> YAEHKSHRGEVSVCDSESLWVTDKSS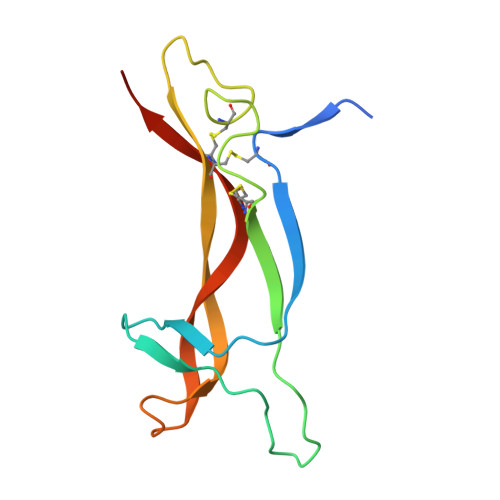AIDIRGHQVTVLGEIKTQNSPVKQYFYETRCKEARPVKNGCRGIDDKHWNSQCKTSQTYVRALTSENNKLVGWRWIRIDTSCVCALSRKIGRT sulfolane | C4 H8 O2 S | 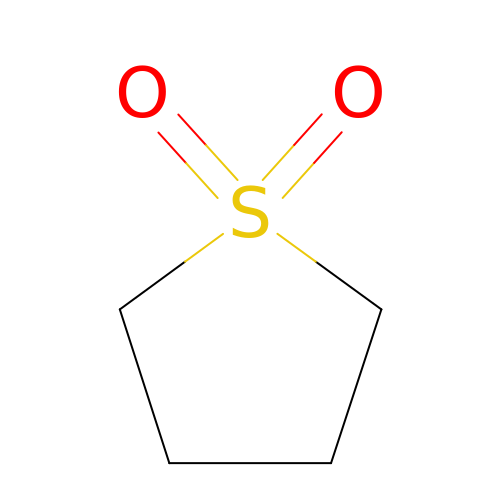HXJUTPCZVOIRIF-UHFFFAOYSA-N>MFVLLVAYALLHIAGCQTTNGLNTSYSVCNGCVGYSENVFAVESGGYIPSDFAFNNWFLLTNTSSVVDGVVRSFQPLLLNCLWSVSGLRFTTGFVYFNGTGRGDCKGFSSDVLSDVIRYNLNFEENLRRGTILFKTSYGVVVFYCTNNTLVSGDAHIPFGTVLGNFYCFVNTTIGNETTSAFVGALPKTVREFVISRTGHFYINGYRYFTLGNVEAVNFNVTTAETTDFCTVALASYADVLVNVSQTSIANIIYCNSVINRLRCDQLSFDVPDGFYSTSPIQSVELPVSIVSLPVYHKHTFIVLYVDFKPQSGGGKCFNCYPAGVNITLANFNETKGPLCVDTSHFTTKYVAVYANVGRWSASINTGNCPFSFGKVNNFVKFGSVCFSLKDIPGGCAMPIVANWAYSKYYTIGSLYVSWSDGDGITGVPQPVEGVSSFMNVTLDKCTKYNIYDVSGVGVIRVSNDTFLNGITYTSTSGNLLGFKDVTKGTIYSITPCNPPDQLVVYQQAVVGAMLSENFTSYGFSNVVELPKFFYASNGTYNCTDAVLTYSSFGVCADGSIIAVQPRNVSYDSVSAIVTANLSIPSNWTTSVQVEYLQITSTPIVVDCSTYVCNGNVRCVELLKQYTSACKTIEDALRNSAMLESADVSEMLTFDKKAFTLANVSSFGDYNLSSVIPSLPRSGSRVAGRSAIEDILFSKLVTSGLGTVDADYKKCTKGLSIADLACAQYYNGIMVLPGVADAERMAMYTGSLIGGIALGGLTSAASIPFSLAIQSRLNYVALQTDVLQENQKILAASFNKAMTNIVDAFTGVNDAITQTSQALQTVATALNKIQDVVNQQGNSLNHLTSQLRQNFQAISSSIQAIYDRLDIIQADQQVDRLITGRLAALNVFVSHTLTKYTEVRASRQLAQQKVNECVKSQSKRYGFCGNGTHIFSLVNAAPEGLVFLHTVLLPTQYKDVEAWSGLCVDGRNGYVLRQPNLALYKEGNYYRITSRIMFEPRIPTIADFVQIENCNVTFVNISRSEL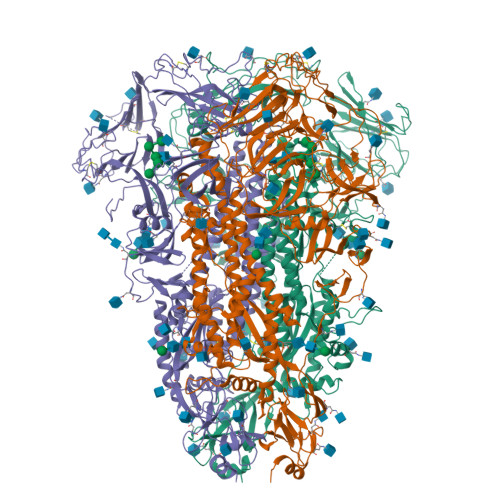QTIVPEYIDVNKTLQELSYKLPNYTVPDLVVEQYNQTILNLTSEISTLENKSAELNYTVQKLQTLIDNINSTLVDLKWLNRVETYIKWPW[3x]>[4x]GSM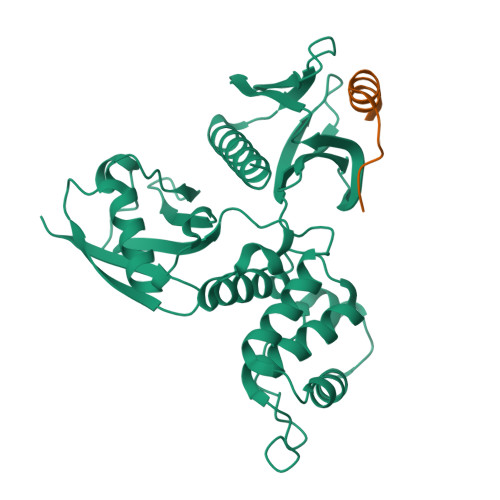PKPINVRVTTMDAELEFAIQPNTTGKQLFDQVVKTVGLREVWFFGLQYVDSKGYSTWLKLNKKVTQQDVKKENPLQFKFRAKFFPEDVSEELIQEITQRLFFLQVKEAILNDEIYCPPETAVLLASYAVQAKYGDYNKEIHKPGYLANDRLLPQRVLEQHKLTKEQWEERIQNWHEEHRGMLREDSMMEYLKIAQDLEMYGVNYFEIKNKKGTELWLGVDALGLNIYEHDDKLTPKIGFPWSEIRNISFNDKKFVIKPIDKKAPDFVFYAPRLRINKRILALCMGNHELYMRRRKPDTIEVQQMKAQAR;>[4x]KEKARAMRVNKRAPQMDWNRKREIFSNF> GPLGSPEFPGGIWNTLLAIHKTEKAVETPKKVFAVANGVLYSVGKEAPHEAKIFDRISGLSDTSVSSIAYSEQLKSLVIYYASGNIDILDEAGRVTNVPALKDNIDLIDKTLNRLLIVGNRAYLAGGFGLSVLDVAEARIPATYAKGTKVTDVAKLDNDRLLMLKEGQLFIGKETDNLQDPAAWTALSLNLPMGSVTGLGIVGEDICFLLADGRVYVAANQSFEPELLLSSSADSRLYVTDRGLFICAENRIYFIEKGRKTTQFPIADVLGVGAMNESNTAYIALGEEGLA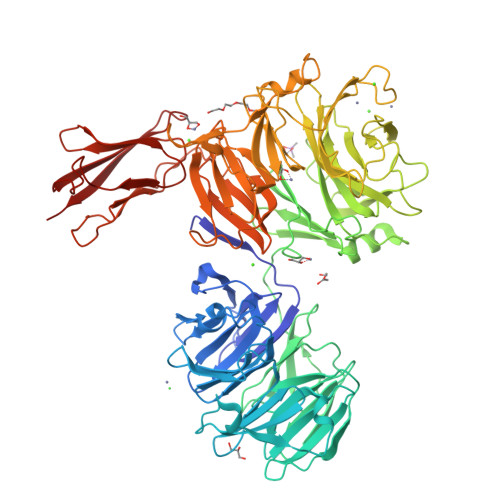SLLLAEGSTAEAMPVAFDGPGDNDFYEMRFSHGRLYAASGLWGTNLMGHAGMVKLYDGNRWTNFDKKTVQEQLGGGFSFNDAIDIAVSNGDPDHFFVGTWGNGLFEFKDGKAIARYSGNETAIAECNPGDARVKAIAFDNKGNLWGTLGAVGKNIFMYDPQSSTWHSFSYPDVANLASFGNMIILPNGDKWVNILHRSGGSTRKGVLIFNDRGTPETTSDDSHLYVEQFVNRLGAAIGHKTIYAMAVDHNGSVWMGSDIGIFGVYNAAGVLSSTSTPIAVRPVGGEEPNLYYVLDKVTVTDIVVDKLNHKWVATQGTGLYLLSEDCSKILAQFTVENSPLLSNNILSLALNDDNGLLYIGTADGLMTFQTGTGSGSASELDGVYVYPNPLRPEYPDGVTIAGLQAGCSVKITDTTGRLLYQTESVTTEVKWNARGADGNRVASGVYAVAVYDPVSKKSKLIRFAVIR>[2x]MDVIREYLMFNELSALSSSPESVRSRFSSIYGTNPDGIALNNETYFNAVKPPITAQYGYYCYKNVGTVQYVNRPTDINPNVILAQDTLTNNTNEPFTTTITITGSFTNTST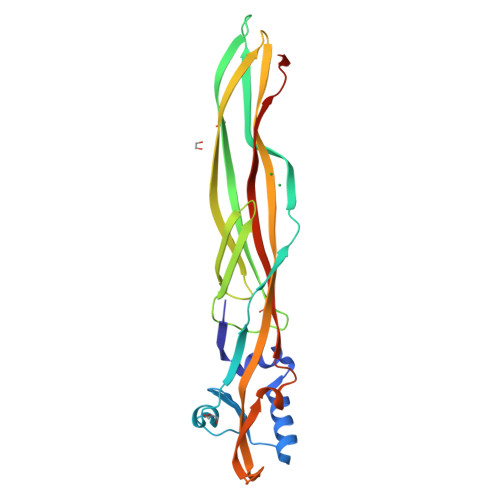VTSSTTTGFKFTSKLSIKKVFEIGGEVSFSTTIGTSETTTETITVSKSVTVTVPAQSRRTIQLTAKIAKESADFSAPITVDGYFGANFPKRVGPGGHYFWFNPARDVLNTTSGTLRGTVTNVSSFDFQTIVQPARSLLDEQ>MTPRSRLATLGTVILLVCFCAGAAHSRGDTFQTSSSPT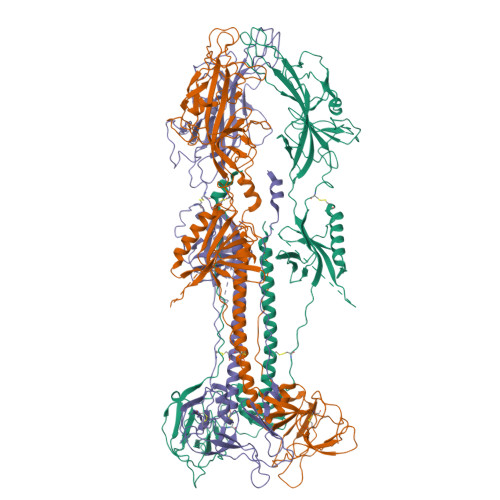PPGSSSKAPTKPGEEASGPKSVDFYQFRVCSASITGELFRFNLEQTCPDTKDKYHQEGILLVYKKNIVPHIFKVRRYRKIATSVTVYRGHRESAITNKYELPRPVPLYEISHMDSTYQCFSSMKVNVNGVENTFTDRDDVNTTVFLQPVEGLTDNIQRYFSQPVIYAEPGRVEATYRVRTTVNCEIVDMIARSAEPYNYFVTSLGDTVEVSPFCYNESSCSTTPSNKNGLSVQVVLNHTVVTYSDRGTSPTPQNRIFVETGAYTLSWASESKTTAVCPLALWKTFPRSIQTTHEDSFHFVANEITATFTAPLTPVANFTDTYSCLTSDINTTLNASKAKLASTHVPNGTVQYFHTTGGLYLVWQPMSAINLTHAQGDSGNPTSSPPPSASPMTTSASRGGSGGASTAAAGGGGSTDNLSYTQLQFAYDKLRDGINQVLEELSRAWCREQVRDNLMWYELSKINPTSVMTAIYGRPVSAKFVGDAISVTECINVDQSSVNIHKSLRTNSKDVCYARPLVTFKFLNSSNLFTGQLGARNEIILTNNQVETCKDTCEHYFITRNETLVYKDYAYLRTINTTDISTLNTFIALNLSFIQNIDFKAIELYSSAEKRLASSGSHHHHHH[3x]> KVFERCELARTLKRLGMDGYRGISLANWMC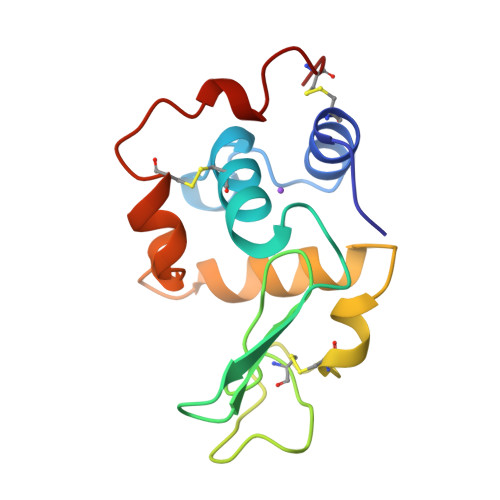LAKWESGYNTRATNYNAGDRSTDYGIFQINSRYWCNDGKTPGAVNAAHLSCSALLQDNIADAVAAAKRVVRDPQGIRAWVAWRNRCQNRDVRQYAQGCGV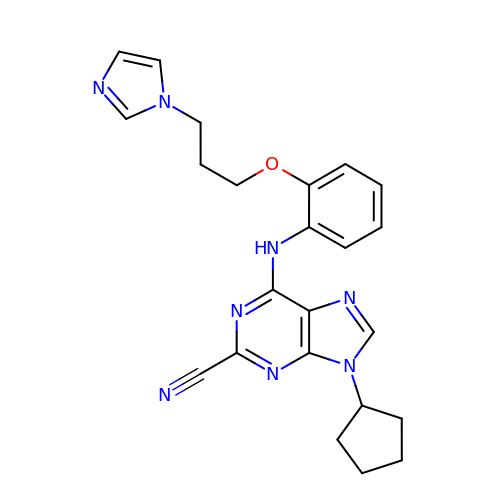9-CYCLOPENTYL-6-[2-(3-IMIDAZOL-1-YL-PROPOXY)-PHENYLAMINO]-9H-PURINE-2-CARBONITRILE | C23 H24 N8 O | JJNKDTWKWYLERH-UHFFFAOYSA-N>[2x]MGASKLRAVLEKLKLSR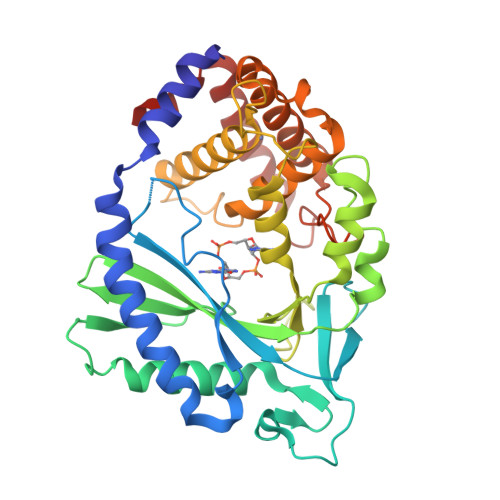DDISTAAGMVKGVVDHLLLRLKCDSAFRGVGLLNTGSYYEHVKISAPNEFDVMFKLEVPRIQLEEYSNTRAYYFVKFKRNPKENPLSQFLEGEILSASKMLSKFRKIIKEEINDIKDTDVIMKRKRGGSPAVTLLISEKISVDITLALESKSSWPASTQEGLRIQNWLSAKVRKQLRLKPFYLVPKHAKEGNGFQEETWRLSFSHIEKEILNNHGKSKTCCENKEEKCCRKDCLKLMKYLLEQLKERFKDKKHLDKFSSYHVKTAFFHVCTQNPQDSQWDRKDLGLCFDNCVTYFLQCLRTEKLENYFIPEFNLFSSNLIDKRSKEFLTKQIEYERNNEFPVFDEF>SEEVVIAGMSGKLPESENLQEFWANLIGGVDMVTDDDRRWKAGLYGLPKRSGKLKDLSKFDASFFGVHPKQAHTMDPQLRLLLEVSYEAIVDGGINPASLRGTNTGVWVGVSGSEASEALSRDPETLLGYSMVGCQRAMMANRLSFFFDFKGPSIALDTACSSSLLALQNAYQAIRSGECPAALVGGINLLLKPNTSVQFMKLGMLSPDGTCRSFDDSGSGYCRSEAVVAVLLTKKSLARRVYATILNAGTNTDGSKEQGVTFPSGEVQEQLICSLYQPAGLAPESLEYIEAHGTGTKVGDPQELNGITRSLCAFRQAPLLIGSTKSNMGHPEPASGLAALTKVLLSLEHGVWAPNLHFHNPNPEIPALLDGRLQVVDRPLPVRGGNVGINSFGFGGSNVHVILQPNTRQAPAPTAHAALPHLLHASGRTLEAVQDLLEQGRQHSQDLAFVSMLNDIAATPTAAMPFRGYTVLGVEGRVQEVQQVSTNKRPLWFICSGMGTQWRGMGLSLMRLDSFRESILRSDEAVKPLGVKVSDLLLSTDERTFDDIVHAFVSLTAIQIALIDLLTSVGLKPDGIIGHSLGEVACGYADGCLSQREAVLAAYWRGQCIKDAHLPPGSMAAVGLSWEECKQR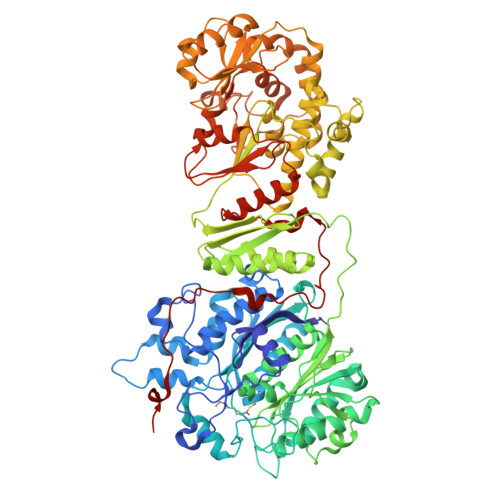CPAGVVPACHNSEDTVTISGPQAAVNEFVEQLKQEGVFAKEVRTGGLAFHSYFMEGIAPTLLQALKKVIREPRPRSARWLSTSIPEAQWQSSLARTSSAEYNVNNLVSPVLFQEALWHIPEHAVVLEIAPHALLQAVLKRGVKSSCTIIPLMKRDHKDNLEFFLTNLGKVHLTGINVNPNALFPPVEFPAPRGTPLISPHIKWDHSQTWDVPVAEDFPN[4x]>AERLCRHCPKDWTFFQGNCYFMSNSQRNWHDSVTACQEVRAQLVVIKTAEEQNFLQLQTSRSNRFSWMGLSDLNQ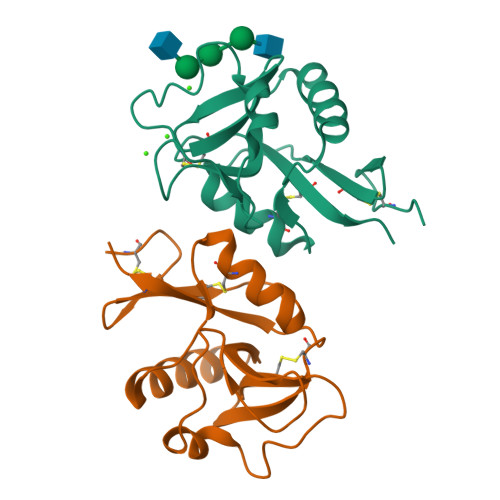EGTWQWVDGSPLSPSFQRYWNSGEPNNSGNEDCAEFSGSGWNDNRCDVDNYWICKKPAACFRDE[2x]The vertebrate Nav channel is composed of an ∼250-kDa α subunit, which contains the ion-selective pore, together with ∼40-kDa β subunits that modulate the voltage sensitivity, gating kinetics, and trafficking of the channel. The Nav β subunits (β1 to β4) are related to the L1 family of cell adhesion molecules and are thought to possess a single extracellular V-type Ig domain, connected via a stalk to an α-helical transmembrane domain and an intracellular carboxyl-terminal region (4–6). The Ig domain contacts the Nav α subunit and modulates its gating properties. Here, we report the crystal structure of the human β3 subunit immunoglobulin (Ig) domain, a functionally important component of Nav channels in neurons and cardiomyocytes.

The structure was determined to a resolution of 2.5 Å, with phases obtained using the molecular replacement method. The β3 Ig domain assembled as a trimer in the asymmetric unit. The β3 subunit protomers in the asymmetric unit are related to each other by a pseudo 3-fold NCS axis. The total buried surface area within the trimer is around 2565 Å2. Potential N-linked glycosylation sites of each protomer point away from the trimer interface. Key features common to all Ig domains are present in the protomer. These include a buried disulfide bond (Cys-21–96) that stabilizes adjacent faces of the molecule and the presence of Ig domain-typical β-sheets. Instead, the region is held in place by a surface intramolecular disulfide bond, Cys-2–24. An intramolecular salt bridge between Glu-4 and Arg-115 further constrains the local conformation of the peptide chain. As a result, the side chains of residues Val-3, Val-5, and Pro-6 are surface-exposed. These residues from each protomer provide the main trimer-stabilizing hydrophobic contacts.

>[3x]VCVEVPSETEAVQGNPMKLRCISCMKREEVEATTVVEWFYRPEGGKDFLIYEYRNGHQEVESPFQGRLQWNGSKDLQDVSITVLNVTLNDSGLYTCNVSREFEFEAHRPFVKTTRLIPLRVHHHHHH>[4x]MPCPVTTFGPKACVLQNPQTIMHIQDPASQRLTWNKSPKSVLVIKKMRDASLLQPFKELCTHLMEENMIVYVEKKVLEDPAIASDESFGAVKKKFCTFREDYDDISNQIDFIICLGGDGTLLYASSLFQGSVPPVMAFHLGSLGFLTPFSFENFQSQVTQVIEGNAAVVLRSRLKVRVVKELRGKKTAVHNGLGEKGSQAAGLDMDVGKQAMQYQVLNEVVIDRGPSSYLSNVDVYLDGHL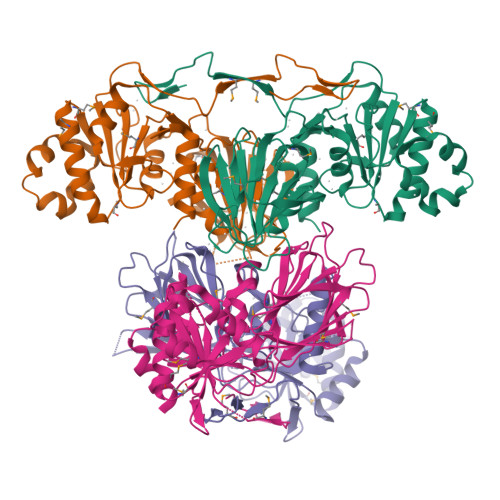ITTVQGDGVIVSTPTGSTAYAAAAGASMIHPNVPAIMITPICPHSLSFRPIVVPAGVELKIMLSPEARNTAWVSFDGRKRQEIRHGDSISITTSCYPLPSICVRDPVSDWFESLAQCLHHHHHH> STRFTEEYQLFEELGKGAFSVVRRCVKVLAGQEYAAMIINTKKLSARDHQKLEREARICRLLKHPNIVRLHDSISEEGHHYLIFDLVTGGELFEDIVAREYYSEADASHCIQQILEAVLHCHQMGVVHRNLKPENLLLASKLKGAAVKLADFGLAIEVEGEQQAWFGFAGTPGYLSPEVLRKDPYGKPVD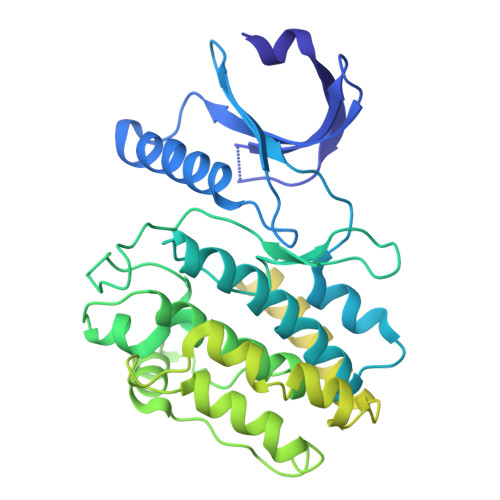LWACGVILYILLVGYPPFWDEDQHRLYQQIKAGAYDFPSPEWDTVTPEAKDLINKMLTINPSKRITAAEALKHPWISHRSTVASCMHRQETVDCLKKFNARRKLKGAILTTMLATRNFSGGKSGGNKKSDGVKESSESTNTTIEDEDTKVRKQEIIKVTEQLIEAISNGDFESYTKMCDPGMTAFEPEALGNLVEGLDFHRFYFENLWSRNSKPVHTTILNPHIHLMGDESACIAYIRITQYLDAGGIPRTAQSEETRVWHRRDGKWQIVHFHRSGAPSVLPH>[2x]DNNCTHFPVGQSHMLLELRTAFSQVKTFFQTKDQ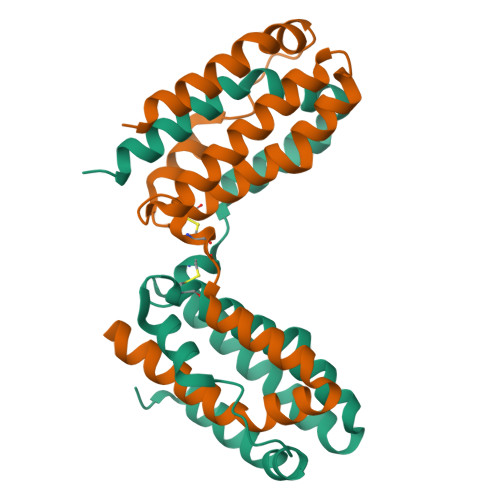LDNILLTDSLMQDFKGYLGCQALSEMIQFYLVEVMPQAEKHGPEIKEHLNSLGEKLKTLRMRLRRCHRFLPCENKSKAVEQVKSDFNKLQDQGVYKAMNEFDIFINYIEAYMMIKMKSLEHHHHHHHH> GPGSMAG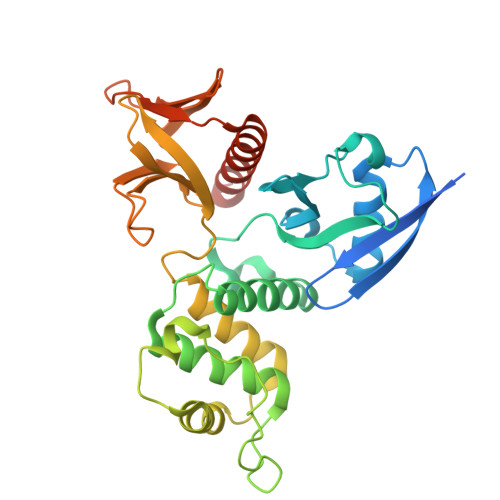AIASRMSFSSLKRKQPKTFTVRIVTMDAEMEFNCEMKWKGKDLFDLVCRTLGLRETWFFGLQYTIKDTVAWLKMDKKVLDHDVSKEEPVTFHFLAKFYPENAEEELVQEITQHLFFLQVKKQILDEKIYCPPEASVLLASYAVQAKYGDYDPSVHKRGFLAQEELLPKRVINLYQMTPEMWEERITAWYAEHRGRARDEAEMEYLKIAQDLEMYGVNYFAIRNKKGTELLLGVDALGLHIYDPENRLTPKISFPWNEIRNISYSDKEFTIKPLDKKIDVFKFNSSKLRVNKLILQLCIGNHDLFMRRRKADSLEVQQ>MIAVKDITDLNIQDIISQLTSEVINGDTTPSSAKFACEINSYIINYNLSNINLINTQLKNTKILYRKGLISKLDYEKYKRYCIISRFKNNIDEFILYFSTNYKDSQSLKIAIKELQNSCSSSLILELPHDYIRKIDVLLTSIDSAIQRSSDLNKTIIKQLNKLRSSLSRYIGYNNVLQKQEITINIKPINKNFELEDISFVSTRNKQYFKHNSLTLKNPHIEKLEVCENIYGINGWLTFDLAYINNHKDFNFLLSPNQPILLDIQINDSFNFYKKESKKDHHKRTTRFIAIGFNSNSIDIHENFEYSIYSYTKNVSSGVKKFKIQFHDPLKALWTKHKPSYIALNKSLDDIFKDNFFFDSLFSLDTNKSNNLKIRIPQAFISTVNRNFYDFFIQQLEQNKCYLKYFCDKKSGKVSYHVVDQVDNDLQRNIVNSDEDLKDKLSPYDISCFKKQILISNKSNFYVKEKNICPDVTLNTQRKEDRKISDTLVKPFSSILKDNLQSVEYIQSNNDDKQEIITTGFEILLTSRNTLPFLDTEITLSKLDNDQNYLLGATDIKSLYISQRKLLFKRSKYCSKQLYENLHNFHYKSDSESDVYEKIAFTKYPSLTHDNSITYKIKDYSNLTPEYPKYKSFSNFYINGRITIGENVNNDSKKAYKFFKNHKPEESSIAEFQENGEKGTSAILNSKADILYAIEIAKEMLSDKSSDKPIIYLPLKVNINSANNQFIPLRNDDIILIEIQSFTKGEIIELISNSAISTKKAQQQLLQRQLLGSKENCEMAYTQTSDSETFSLTQVNEDCENSFLINDKKGIFLRYKSKGN[3x];>MDYKDDDDKDYKDDDDKDYKDDDDKGSKADHIFNLEEQGLLIDIKDDSKGCTTKLESSGKITHNATESIESSADKQIIENVKDSKISITEKEILLATKKSSIMLSEDKIV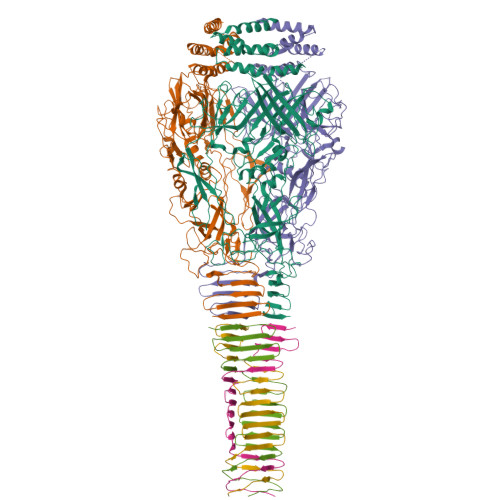IKIGNSLIILDDSNISLESATINIKSSANINIQASQNIDIKSLNNSIKADVNLNAEGLDVNIKGSVTASIKGSAATMVG[3x]6-{[(1R)-1-(4-chlorophenyl)ethyl]amino}-1-cyclopentyl-1,5-dihydro-4H-pyrazolo[3,4-d]pyrimidin-4-one 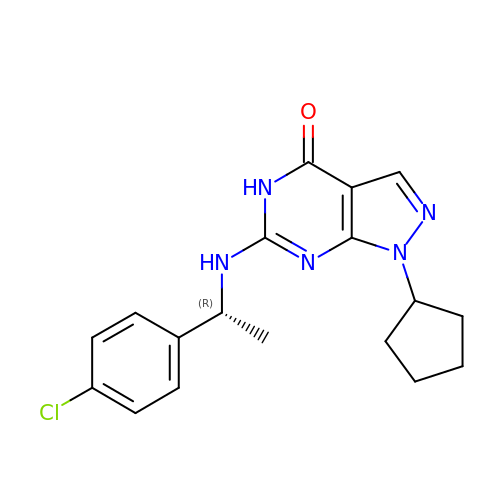| C18 H20 Cl N5 O | FIUCLBJMUGCQTF-LLVKDONJSA-N>[4x]SMASHHHHHHSSGDYKDDDDKLEVLFQGPSGAASRRRYLLYDVNPPAGFNLRRDVYI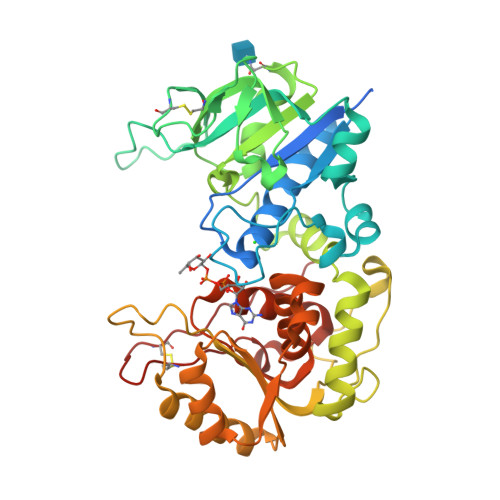RIASLLKTLLKTEEWVLVLPPWGRLYHWQSPDIHQVRIPWSEFFDLPSLNKNIPVIEYEQFIAESGGPFIDQVYVLQSYAEGWKEGTWEEKVDERPCIDQLLYSQDKHEYYRGWFWGYEETRGLNVSCLSVQGSASIVAPLLLRNTSARSVMLDRAENLLHDHYGGKEYWDTRRSMVFARHLREVGDEFRSRHLNSTDDADRIPFQEDWMKMKVKLGSALGGPYLGVHLRRKDFIWGHRQDVPSLEGAVRKIRSLMKTHRLDKVFVATDAVRKEYEELKKLLPEMVRFEPTWEELELYKDGGVAIIDQWICAHARFFIGTSVSTFSFRIHEEREILGLDPKTTYNRFCGDQEKACEQPTHWKITY>[3x]MSVEKIPGYTYGETENRAPFNLEDLKLLKEAVMFTAEDEEYIQKAGEVLEDQVEEILDTWYGFVGSHPHLLYYFTSPDGTPNEKYLAAVRKRLSRWILDTSNRSYDQAWLDYQYEIGLRHHR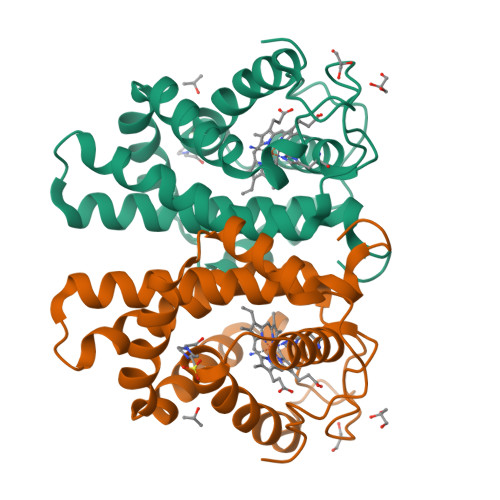TKKNQTDNVESVPNIGYRYLVAFIYPITATMKPFLARKGHTPEEVEKMYQAWFKATTLQVALWSYPYVKYGDF> CQPIFLNVLEAIEPGVVCAGHDNNQPDSFAALLSSLNELGERQLVHVVKWAKALPGFRNLHVDDQMAVIQYSWMGLMVFAMGWRSFTNVNSRMLYFAPDLVFNEYRMHKSRMYSQCVRMRHLSQEFGWLQITPQEFLCMKALLLFSIIPVDGLKNQKFFDELRMNYIKELDRIIACKRKNPTSCSRRFYQLTKLLDSVQPIARELHQF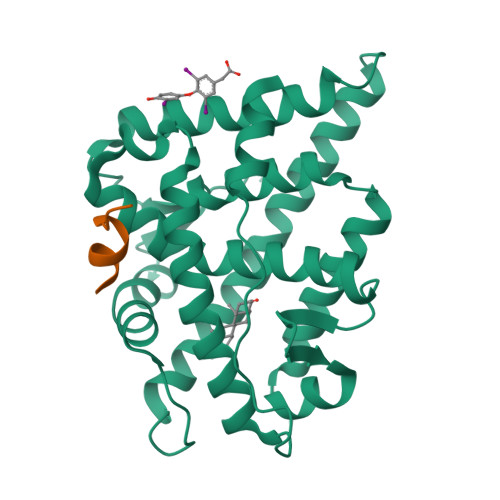TFDLLIKSHMVSVDFPEMMAEIISVQVPKILSGKVKPIYFHTQ;> LLRYLLDKDD> SMQELQGLDYCKPTRLDLLLDMPPVSYDVQLLHSWNNNDRSLNVFVKEDDKLIFHRHPVAQSTDAIRGKVGYTRGLHVWQITWAMRQRGTHAVVGVATADAPLHSVGYTTLVGNNHESWGWDLGRNRLYHDGKNQPSKTYPAFLEPDETFIVPDSFLVALDMDDGTLSFIVDGQYMGVAFRGLKGKKLYPVVSAVWGHCEIRMRYLNGLDPE;> NELNNNLPGGA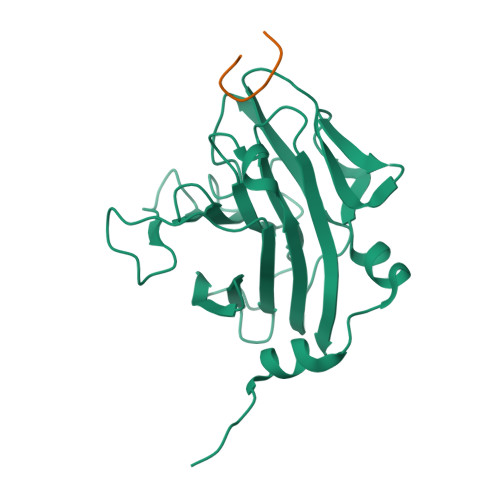PAAP Type III secretion systems (T3SSs) are membrane-embedded nanomachines that export dedicated proteins from the bacterial cytoplasm. FliD and FliC are found in complex with their dedicated chaperones FliT and FliS, respectively, in the cytoplasm. Here we report the structures of the ternary complexes among the FliD and FliC flagellar proteins, their cognate chaperones FliT and FliS, and the export gate protein FlhAC. FlhAC folds in a clamp-like structure with four discrete subdomains (d1 through d4).

Several constructs were tested and the highest quality NMR spectra suitable for solution structure determination were provided by a ternary complex formed between FlhAC and a fused FliT−FliDC construct, wherein FliDC consists of the last 40 C-terminal residues of FliD. The ternary complex was readily crystallized and the X-ray crystallographic structure of the FlhAC−FliT−FliDC ternary complex was determined at 2.75 Å resolution. The solution and crystal structures are essentially identical. Two distinct interfaces mediate the formation of the ternary complex. In the major interface, which buries a total surface of 350 Å2, the FliT helix α4 juxtaposes with a hydrophobic cleft of FlhAC located between domains d1 and d2. Two bulky non-polar residues, Leu102 and Tyr106, emanating from FliT helix α4 bury their side chains into the FlhAC hydrophobic dimple. In addition to a network of intimate non-polar contacts, FliT Tyr106 forms an optimal hydrogen bond with the side chain of FlhAC Asp456 (O–H⋯O distance 2.3 Å). Amino acid substitutions that perturbed the binding interface decreased the ternary complex stability, with FliT residues Leu102 and Tyr106 and FlhA residues Asp456 and Leu461 being essential for complex formation. The minor binding interface features a salt bridge between FliT Arg98 and FlhA Glu640. To maximize the binding interface with FlhAC, FliT undergoes a dramatic conformational change with helices α3 and α4 merging to one continuous, long α helix.

>GEDSLGMEVGYRLIPMVDFQQDGELLGRIRSIRKKFAQDMGFLPPVVHIRDNMDLQPARYRILMKGVEIGSGDAYPGRWLAINPGTAAGTLPGEKTVDPAFGLDAIWIESALKEQAQIQGFTVVEASTVVATHLNHLIGQFSAELFGRQEAQQLLDRVSQEMPKLTEDLVPGVVTLTTLHKVLQNLLAEKVPIRDMRTILETLAEHAPLQSDPHELTAVVRVALGRAITQQWFPGNEEVQVIGLDTALERLLLQALQGGGGLEPGLADRLLAQTQEALSRQEMLGAPPVLLVNHALRPLLSRFLRRSLPQLVVLSNLELSDNRHIRMTATIGGK[3x];>GAHMSIDETVARYKAQFTQLDTMMSKLNNTSSYLTQQFTAMNKSGGSGGSGSGGSGGMTSTVEFINRWQRIALLSQSLLELAQRGEWDLLLQQEVSYLQSIETVMEKQTPPGITRSIQDMVAGYIKQTLDNEQLLKGLLQQRLDELSSLIGQSTRQKSLNNAYGRLSGMLLVPDAPGAS[3x]> ASAKLPGDFGPPRGEPIHAVLTSPPLVPPPVNRTYPAKVIVELEVVEKEMQISEGVSYTFWTFGGTVPGSFIRVRQGDTVEFHLKNHPSSKAPHNIDLHGVTGPGGGAASSFTAPGHESQFTFKALNEGIYVYHCATAPVGMHIANGMYGLILVEPPEGLPKVDHEYYVMQGDFYTAGKYREKGLQPFDMEKAIDERPSYVLFNGAEGALTGDKALHAKVGETVRIFVGNGGPNLVSSFHVIGAIFDQVRYEGGTNVQKNVQTTLIPAGGAAVVKFTARVPGSYVLVDHSIFRAFNK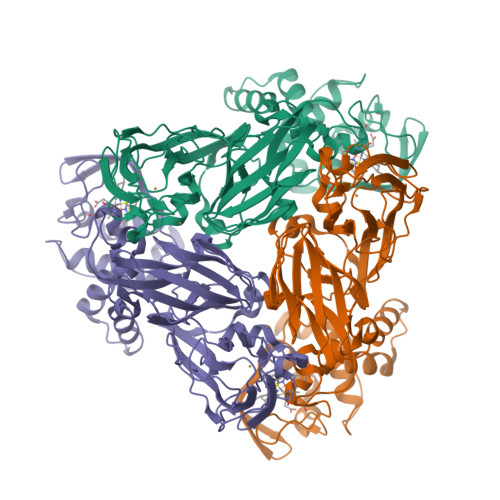GAMAILKIDGAENKLVYSGKELDSVYLGDRAAPNMSAVTKATQASVSGTLTVQDQVQAGRALFAGTCSVCHQGNGAGLPGVFPPLAKSDFLAADPKRAMNIVLHGLNGKIKVNGQEYDSVMPPMTQLNDDEVANILTYVLNSWDNPGGRVSAEDVKKVRAQPAPAKAVAEH>[2x]MRGSHHHHHHGSMSELITENMHMKLYMEGTVNNHHFKCTSEGEGKPYEGTQTMRIKVVEGGPLPFAFDILATSFMYGSKTFINHTQGIPDF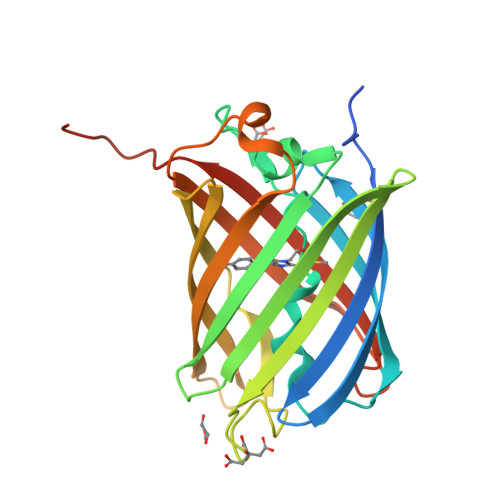FKQSFPEGFTWERVTTYEDGGVLTATQDTSLQDGCLIYNVKIRGVNFPSNGPVMQKKTLGWEASTEMLYPADGGLEGRSDMALKLVGGGHLICNLKTTYRSKKPAKNLKMPGVYYVDRRLERIKEADKETYVEQHEVAVARYCDLPSKLGHKLN>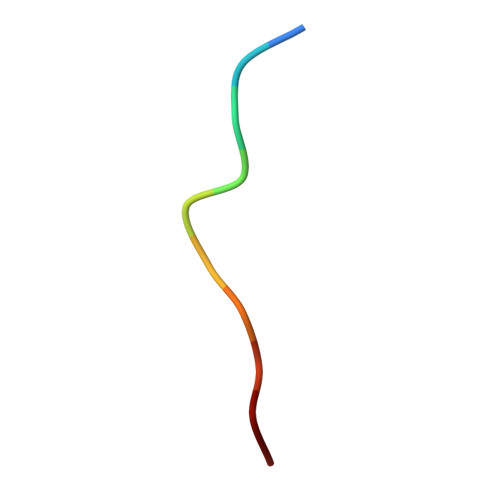 PKRPTTLNLF>[2x]SNAMTPMPVTIELAVAKTHKFGTRESGDTVELVERPGGGFSAVLVDGQGSGAGAKRLSLLVAGAAVRLLNEGVRDGAAARAAHDFLYA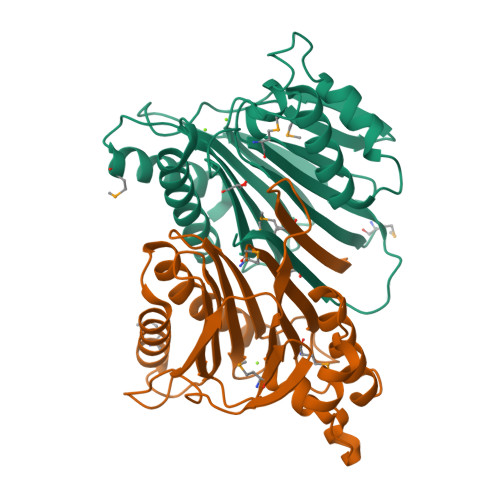MRDGKVSAALDILSVDLASRSVLVTRNSEVPMLLGRNGEFEQISESGGRIGIYRHTRPRVLEFPAEPGLTVILVSDGIIGAGGRRGQPLEFLATGGRVAGPETPAQAIADELLEAALVADDGRAGDDMTVVVLRLRNVEEVEPIRRMALTVPLG N-{3-[(furan-2-carbonyl)amino]phenyl}-2,3-dihydro-1,4-benzodioxine-6-carboxamide | C20 H16 N2 O5 | 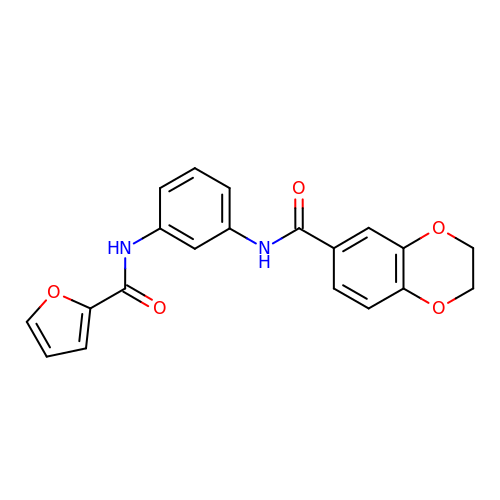QWGFUNDUGLPNFS-UHFFFAOYSA-N>MERQNIHNFGAMAKEVIEATAKAVNNFWEGLSILEISHRSKEWINVMNETKALMKEVMDIPEGYEILFFGGGASLQFLMVAMNLLNKKACYLDTGVWASKAIKEAENIGEVKIIGTSKDKNYTYIPEYQIPSDYDYFHITTNNTIYGTEIRKDIESPIPLVADMSSD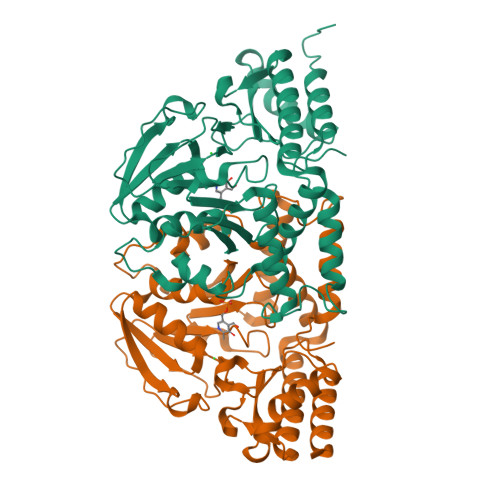ILSKPIDISKYSLIYAGAQKNCGAAGVTIVIIKKEILGKVQRKIPIILDYQVHILNNSMYNTPPVISIFTVNQTLKYIKKIGGLKKIQELNEEKARLLYAEIDRNKIFRGTVRKKDRSIMNVCFVMEEQYKQLENEFSEYALQKGIIGIKGHRSVGGFRASIYNAVTIESVQALIKCMHDFEQLHTH[2x]>[6x]SNAMDKTISVIGMPMDLGQARRGVDMGPSAIRYAHLIERLSDMGYTVEDLGDIPINREKIKNDEELKNLNSVLAGNEKLAQKVNKVIEEKKFPLVLGGDHSIAIGTLAGTAKHYDNLGVIWYDAHGDLNTLETSPSG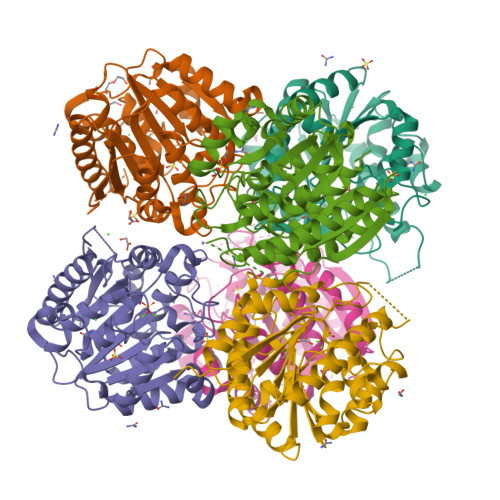NIHGMPLAVSLGIGHESLVNLEGYAPKIKPENVVIIGARSLDEGERKYIKESGMKVYTMHEIDRLGMTKVIEETLDYLSACDGVHLSLDLDGLDPNDAPGVGTPVVGGISYRESHLAMEMLYDAGIITSAEFVEVNPILDHKNKTGKTAVELVESLLGKKLL>[2x]GPGSEFHKGSFKDDPQLYQEIRERGLNTSHESDDDILDETTIVVKSYRPAQLTWSQLPEVLESGVLDTLSTEERKRQEAIFEILTSEFSYLHSLSILVTEF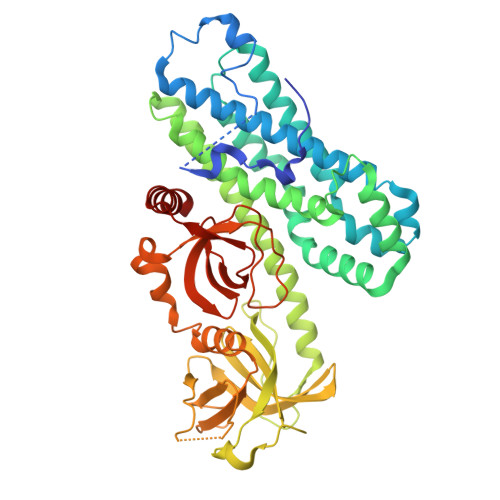LQSRELRATMTQTEHHHLFSNILDVMSASQKFFEALEQRHKAQVCVEDISDILEDHAQHHFHPYIAYCSNEVYQQRTLQKLSNSNAAFRDVLKEIEKRPACGGLPMISFLILPMQRVTRLPLLTDTLCLKTQGHPERYKAASQALKAISKLVKQCNEGAHKMERTEQIYTLNMQLDFGKVKSLPLISASRWLLKRGELFLLEESSIFRKIASRPTCYLFLFNDVLVVTKKKSEESYLVQDYAQLDHVQVRKLEPSEPLLPGGSSRSSSVPYPFQVNLLHNSEGRQEQILLSSDSASDRARWITALTYKERQWQGITNKGELPQVEVTKAYFAKQADEITLQQADIVLVLQEEDGWLHGERLRDGETGWFPESFAHSITSRVAVEGNVRRMERLRVETDV>MGSSHHHHHHSSFLVPRGSHMSQGRKAAERLAKKTVLITGASAGIGKATALEYLEASNGDMKLILAARRLEKLEELKKTIDQEFPNAKVHVAQLDITQAEKIKPFIENLPQEFKDIDILVNNAGKALGSDRVGQIATEDIQDVFDTNVTALINITQAVLPIFQAKNSGDIVNLGSIAGRDAYPTGSIYCASKFAVGAFTDSLRKELINTKIRVILIAPG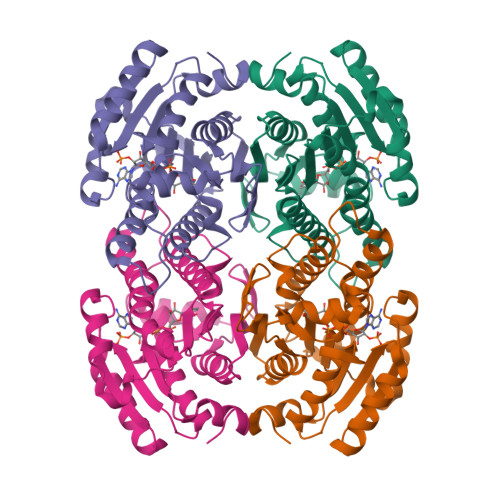LVETEFSLVRYRGNEEQAKNVYKDTTPLMADDVADLIVYATSRKQNTVIADTLIFPTNQASPHHIFRG[4x]> MHHHHHHGSGMALAIKKRVGTYVETVDGSPPVKKLRLQTLAADAKGGKSGKVGNVERKLTALNQLDAYVGNLPAGALVLPTGTPVASTGAPS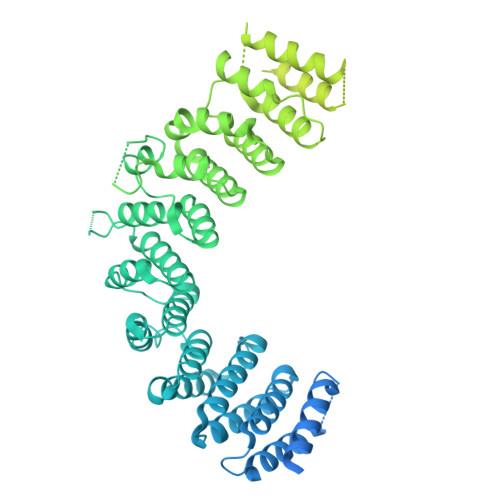TGVIGNPPAAATGAPPMTAANSRELLELLVKITDEISYEDVEMGELKEVASKIFQLYQLQERDSDTSIRVKLLELLSGLGCECATEQALTMIIDYFIFLLRKEVSQKVLAQGMMCLFRIGERRKHMLPISYKTQVAHLAKEQLRSGSAHTQKNAMLVIGRFATKMEGERHYVWKLAFYIDSQDSSVRAQALHALLTLGERGSQLPAVLYKRAVEAMKDDYECVRKEALQLVFMLGNRHPDYILPSDRQQEELRMIDAAFSKVCEALCDLSLQIRVLAAELLGGMTAVSREFLHQTLDKKLMSNLRRKRTAHERGARLVASGEWSSGKRWADDAPQEHLDAQSISIIASGACGALIHGLEDEFLEVRTAAVASMCKLALSRPDFAVTSLDFLVDMFNDEIEDVRLKAIYSLTAIAKHIVLREDQLEIMLGSLEDYSVDVREGLHLMLGACRVSTQTCLLMVVQKLLDVLAKYPQDRNSTYACMRKIGQKHPHLVMAVAVHLLYVHPFFETPERDVEDPAYLCVLILVFNAAEHLVPIISLLPTATHRHYAYLRDSMPNLVPQLPIEGASSASATHRIDSAMHQAGSSAEYLQMILSHIEEIFTMTDERLELLQTAQSNLQRLGSIDAGMYGTSNFLETFLAAQIQIEQMQRCASTQRSRVPLKESLAALIRNCLKLQHTFSGLNYGDILQVKQLRLRACALHLVLVVRDRSQSALGPCQMLLQTAGDISEFIKANTKDEEEKPPVVETDMPMKESVSRDAQPDSFTRQLLIKLDGISDPKPGRVFREILPLVQQAPPLALPPANDKIRRCVANILEPCPLQSQDNVIKVTAGLIAAVPFVAEIDNLLESQKADMRIKIKYPDQHMHTVVPKQSDFKPIMTEQGEHKTNVRLRTTILLSHSVWTESSLVEIQLCLAVRPGSELELCKPAKVLFAPKPVRRGI> APDTSVSNKQNFSTDVIYQIFTDRFSDGNPANNPTGAAFDGTCTNLRLYCGGDWQGIINKINDGYLTGMGVTAIWISQPVENIYSIINYSGVNNTAYHGYWARDFKKTNPAYGTIADFQNLIAAAHAKNIKVIIDFAPNHTSPASSDQPSFAENGRLYDNGTLLGGYTNDTQNLFHHNGGTDFSTTENGIYKGLYDLADLNHNNSTVDVYLKDAIKMWLDLGIDGIRMDAVKHMPFGWQKSFMAAVNNYKPVFTFGEWFLGVNEVSPENHKFANESGMSLLDFRFAQKVRQVFRDNTDNMYGLKAMLEGSAADYAQVDDQVTFIDNHDMERFHASNANRRKLEQALAFTLTSRGVPAIYYGTEQYMSGGTDPDNRARIPSFSTSTTAYQVIQKLAPLRKCNPAIAYGSTQERWINNDVLIYERKFGSNVAVVAVNRNLNAPASISGLVTSLPQGSYNDVLGGLLNGNTLSVGSGGAASNFTLAAGGTAVWQYTAATATPTIGHVGPMMAKPGVTITIDGRGFGSSKGTVYFGTTAVSGADITSWEDTQIKVKIPAVAGGNYNIKVANAAGTASNVYDNFEVLSGDQVSVRFVVNNATTALGQNVYLTG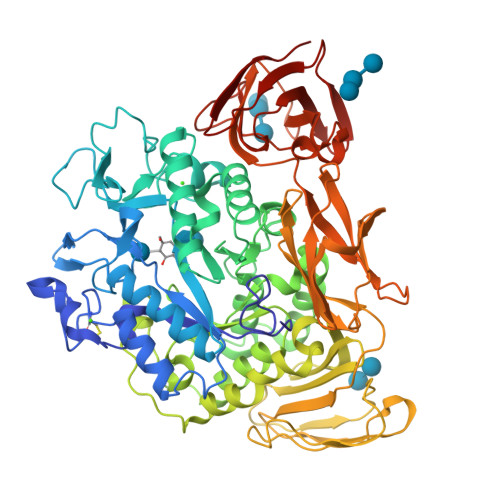SVSELGNWDPAKAIGPMYNQVVYQYPNWYYDVSVPAGKTIEFKFLKKQGSTVTWEGGSNHTFTAPSSGTATINVNWQP> MGSSHHHHHHSSGLVIRGSHMRIALMQHTARPLDPQHNLDLIDDAAARASEQGAQLLLTPELFGFGYVPSQICAQVSAEQVDAARSRLRGIARDRGIALVWSLPGPEGPEQRGITAELADEHGEVLASYQKVQLYGPEEKAAFVPGEQPPPVLSWGGRQLSLLVCYDVEFPEMVRAAAARGAQLVLVPTALAGDETSVPGILLPARAVENGITLAYANHCGPEGGLVFDGGSVVVGPAGQPLGELGVEPGLLVVDLPDQSQDAGSDSADYLQDRRAELHRNW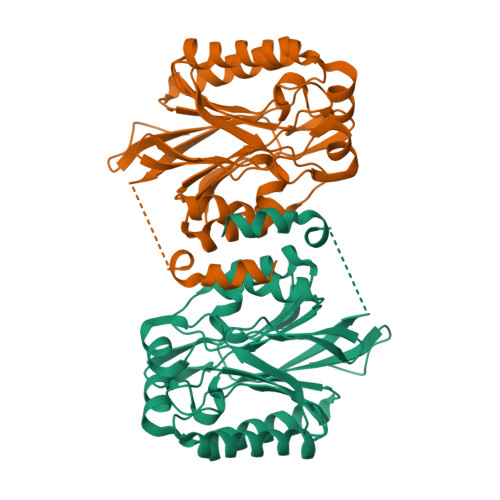L> TDAMTESQPKQTGTRRNSKL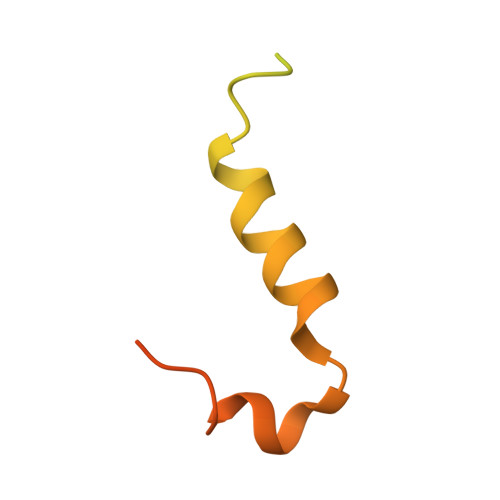LNTKSIQIDEETENSESIASSNTYKEERSNNLLTPQPTNFTTKRLWSEITESMSYLPDPILKNFLSYESLKKRKIHNGRE> MVLGEVYLKDILRTPPTGAIPANVPHPFQTSFY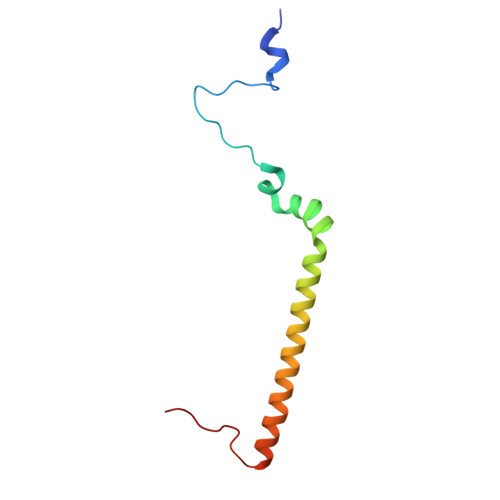TYATKKLIPRHWYLLGGFTFTITLYGILDGLRDSGKKKAYDEAIHAGKTPYTAGGH>MSKGTTSQDAPFGTLLGYAPGGVAIYSSDYSSLDPQEYEDDAVFRSYIDDEYMGHKWQCVEFARRFLFLNYGVVFTDVGMAWEIFSLRFLREVVNDNILPLQAFPNGSPRAPVAGALLIWDKGGEFKDTGHVAIITQLHGNKVRIAEQNVIHSPLPQGQQWTRELEMVVENGCYTLKDTFDDTTILGWMIQTEDTEYSLPQPEIAGELLKISGARLENKGQFDGKWLDEKDPLQNAYVQANGQVINQDPYHYYTITESAEQELIKATNELHLMYLHATDKVLKDDNLLALFDIPKILWPRLRLSWQRRRHHMITGRMDFCMDERGLKVYEYNADSASCHTEAGLILERWAEQGYKGNGFNPAEGLINELAGAWKHSRARPFVHIMQDKDIEENYHAQFMEQALHQAGFETRILRGLDELGWDAAGQLIDGEGRLVNCVWKTWAWETAFDQIREVSDREFAAVPIRTGHPQNEVRLIDVLLRPEVLVFEPLWTVIPGNKAILPILWSLFPHHRYLLDTDFTVNDELVKTGYAVKPIAGRCGSNIDLVSHH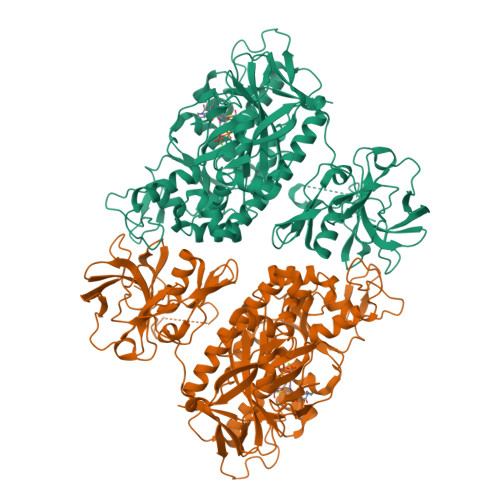EEVLDKTSGKFAEQKNIYQQLWCLPKVDGKYIQVCTFTVGGNYGGTCLRGDESLVIKKESDIEPLIVVKK[2x]>[4x]MSNCQYKIYPPLGIARVGNGPAIKPLSLSTPEVPWAHLYDTNVQYLVTQQELEQLLEEAFGGNVINEISQIKTKLDERKAEKFKQEEIETITGLLGLSHLVPQQQLSRSLDNLELKSTKDSDDIVQQIKGALLKVLSDHYLHAVKKQAQNFYIY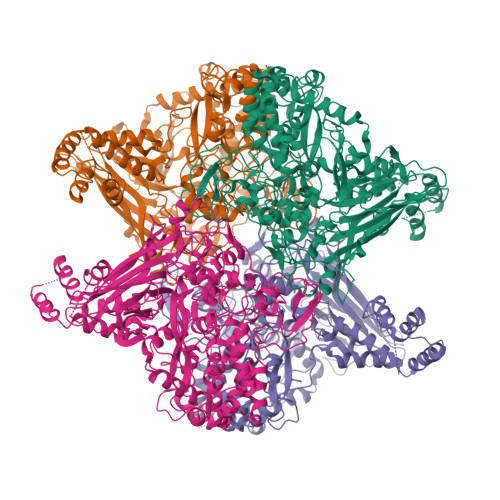KCDEQGNPVEKLKLTDGDKVTWRVEVANKKSFWYDYNNALDLSLHTQGSGNLSKNVSKHRLAPAMTAKRRNPNVITNSLRKQLVISSQGSVSSDNNTQVPLRGKFPANEPDTNNRLSDLLNLQERHNVLQGSIECDNEGVLRFYAGNGISQALSPSSLNTDFADNSNWFDDICDGRVTAVVELKNGDTFEIQDEQSSAWVATTPPDYAPQIEPIVTMYDMVSGAALKEQDLDNLTTQFSDVFPILYRLYRMQWVNQADFTDNAVNTQIRELNSELGFAQLLDNSASAKSLREGIFNQFRNPLFDQDIDVDDPGQSSNEWVSNSRIIPSKDETNIAAKPATSSLKLPFYPNDGIDYPGSPVQWFAIPPFMYQHLQNWAAGDFSVTQVEKESANTIEELGLFYSEQFKNSPNSALLCARGALDALYGGGFHPGVELTWPMRHNLIYSQNDYVSSVTPEINLLGLREFRLKQDLQGLNSPNMYQDFGHVIAVDNVTASIDPNSDAAWLWRSTPGDLTKWMGIPWQSAAASCQAVYTPEDFPIPSWWAANLPVHVLPLARYNKFKDSQSADLPEINGMTHSIAQGMSEETFEHLRLEQFSQRLDWLHTADLGFVGYHAEGGYTNGLIQMVSQWKNMAMVMARPVENPGSSGIPNVVYVAYSQADKD(2S)-sulfonatepropionyl-amino(dethia)-CoA | C24 H41 N8 O20 P3 S 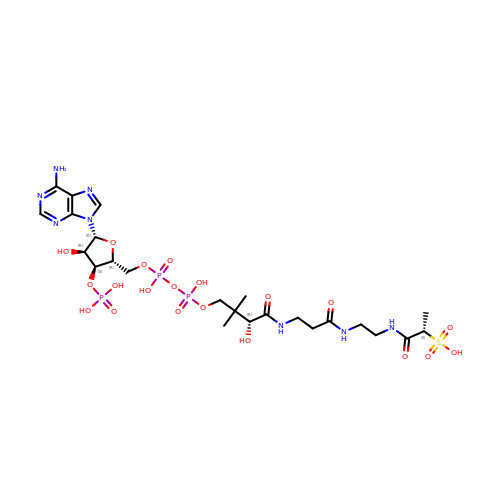| IUFNAUQYWOGJPI-CLSLWNEHSA-N2-acetamido-2-deoxy-alpha-D-glucopyranose 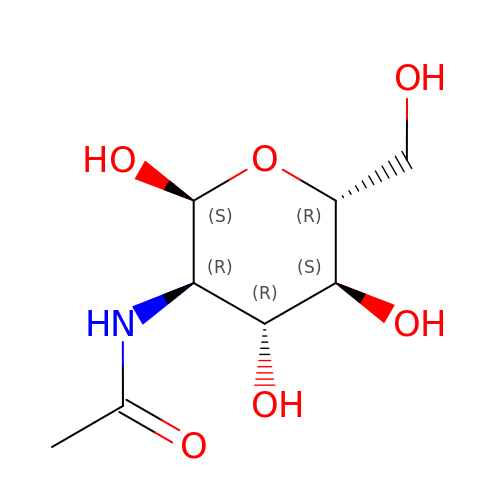| C8 H15 N O6 | OVRNDRQMDRJTHS-PVFLNQBWSA-N> MATTCRTADGDMLDSLCYHVY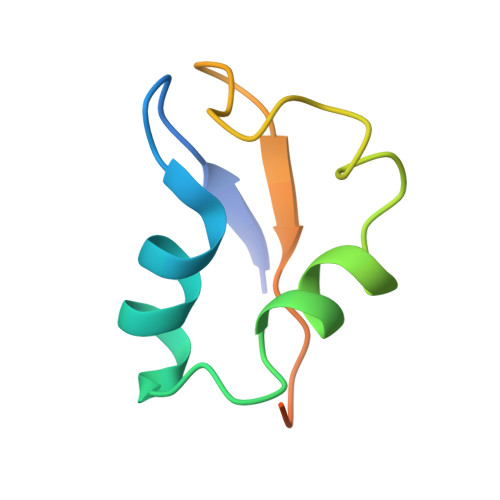GHLLGCVEATLDANPGLADEQQPFRAGLLISFPDMPVVNVEQVRLWD>MVHEEDFKEGYILGFIEAEGSFSVSIKFQRDVFGGVRLDPVFSITQKNREVLEAIKEHLGIGRIMEKAGQPNTYVYVVDNFNELVKLINFLNKYADFMIVKKRQFLMFREIANGLVNGEHLHINGLKRLVKLAYELTKESEKGYRKYDLNHVLSIIDKWDLG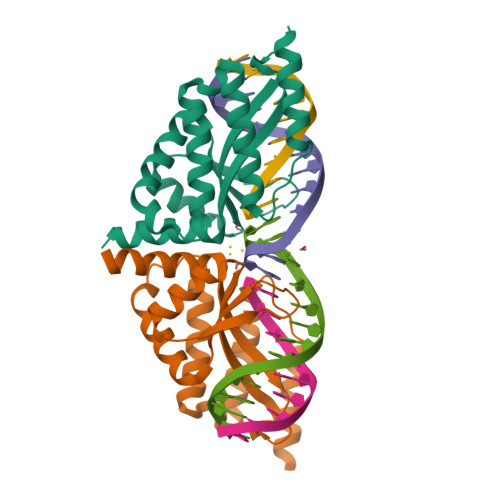RNVSTSL[2x]BZU3 encodes a UDP-Glc 4-epimerase and plays a key role in controlling cell wall synthesis during the morphogenesis of maize stomata. It also catalyzes epimerization of UDP-N-acetylgalactosamine (UDP-GalNAc) to UDP-N-acetylglucosamine (UDP-GlcNAc), regulating N-glycosylation patterns of many proteins that may be involved in cell wall synthesis and signaling pathways. BZU3 formed a homo-dimer, with each protomer folded into two distinct structural units, the N-terminal NAD+ binding domain (residues 1-189) and the C-terminal sugar-binding domain (residues 190-355). The catalytic site was located in the cleft between these two structural domains.

To further address the molecular functions of BZU3, we solved the 3-D structures of the BZU3 protein, both in apo form and in complexes with NAD+/UDP-Glc and NAD+/UDP-GlcNAc, at resolutions of 2.6 Å, 1.25 Å, and 2.15 Å respectively. The flexible sugar moiety was held in place in the vicinity of the catalytic triad of Ser-Tyr-Lys (S133/Y157/K161). S133 forms a bifurcated contact with the sugar moiety of the substrate, whereas both Y157 and K161 directly interact with the ribose moiety of NAD+. Drawing on the structural model, we designed mutations within the conserved catalytic triad and found that S133A significantly reduced catalytic activity, while Y157F completely abolished the inter-conversion between UDP-Glc and UDP-Gal, and UDP-GlcNAc and UDP-GalNAc. Consistent with this result, the transgene of BZU3pro:BZU3Y157F-YFP failed to rescue the stomatal phenotype in bzu3-2. Taken together, these observations imply that the catalytic activity of BZU3 is required for the morphogenesis of maize GCs. With UDP-Gal as substrate, the Km (Michaelis–Menten constant), Vmax (the maximum reaction velocity), and Kcat/Km were 1.45 mM, 1.41 mM·min−1, and 650.3 s−1·mM−1 respectively. Km, Vmax, and Kcat/Km were 2.67 mM, 0.69 mM·min−1, and 172.4 s−1·mM−1, respectively, when using UDP-Glc as substrate. Our biochemical data indicated that the epimerase activity of BZU3 prefers to catalyze conversion of UDP-Gal to UDP-Glc.

>[2x]MVSAVLRTILVTGGAGYIGSHTVLQLLQQGFRVVVVDNLDNASEAALARVAELAGHDGANLVFHKVDLRDRHALVDIFSSHRFEAVIHFAGLKAVGESVHKPLLYYDNNLVGTITLLEVMAANGCKKLVFSSSATVYGWPKEVPCTEEFPLCATNPYGRTKLVIEDICRDVHRSDPDWKIILLRYFNPVGAHPSGYIGEDPCGVPNNLMPYVQQVAVGRLPHLTVYGTDYSTKDGTGVRDYIHVVDLADGHIAALRKLYEDSDKIGCEVYNLGTGKGTSVLEMVAAFEKASGKKIPLVFAGRRPGDAEIVYAATAKAEKELKWKAKYGIEEMCRDLWNWASKNPYGYAGSRDNSK>[16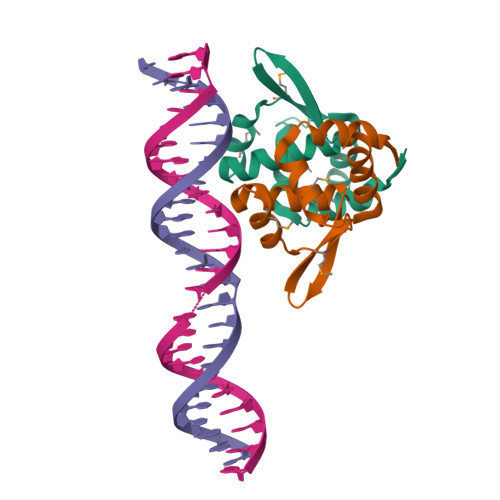x]MNRDHFYTLNIAEIAERIGNDDCAYQVLMAFINENGEAQMLNKTAVAEMIQLSKPTVFATVNSFYCAGYIDETRVGRSKIYTLSDLGVEIVECFKQKAMEMRNL[(3~{S},4~{R})-4-(2-azanyl-6-oxidanylidene-1~{H}-purin-9-yl)pyrrolidin-3-yl]oxymethylphosphonic 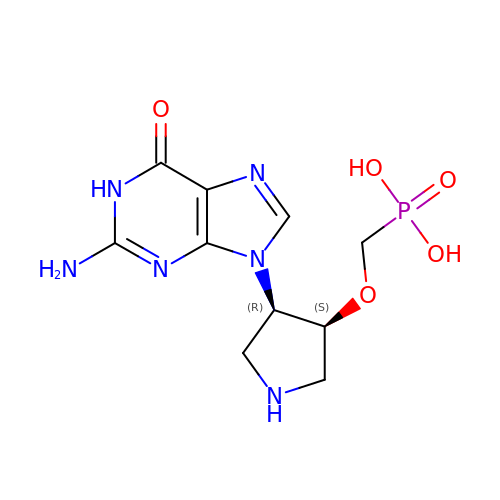acid | C10 H15 N6 O5 P | LMOOKHOOULQCAZ-RITPCOANSA-N> MNVQDRRRLLGPAAAKPMAFSNTTTHVPEKKSTDLTPKGNESEQELSLHTGFIENCNGSALVEARSLGHQTSLITAVYGPRSIRGSFTSQGTISIQLKNGLLEKYNTNELKEVSSFLMGIFNSVVNLSRYPKSGIDIFVYLTYDKDLTNNPQDDDSQSKMMSSQISSLIPHCITSITLALADAGIELVDMAGAGEANGTVVSFIKNGEEIVGFWKDDGDDEDLLECLDRCKEQYNR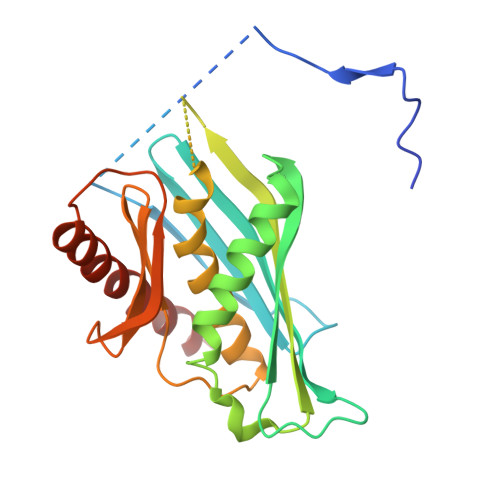YRDLMISCLMNQET tert-butyl 7-amino-3,4-dihydroisoquinoline-2(1H)-carboxylate | C14 H20 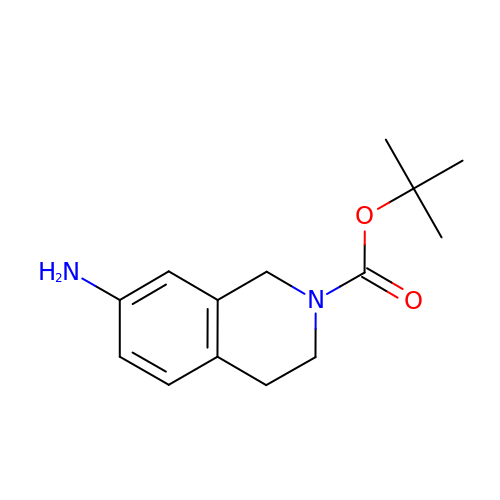N2 O2 | AGRBXKCSGCUXST-UHFFFAOYSA-N>[12x]PLIRIDLTSDRSREQRRAIADAVHDALVEVLAIPARDRFQILTAHDPSDIIAEDAGLGFQRSPSVVIIHVFTQAGRTIETKQRVFAAITESLAPI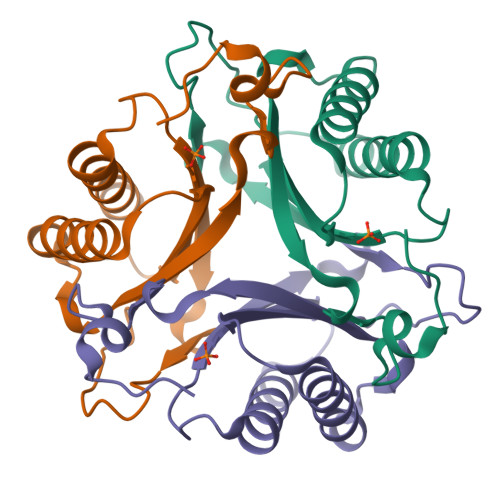GVAGSDVFIAITENAPHDWSFGFGSAQYVTGELAIPATGAA>DFALPINFGADIEYTTGANSVPFEVVTNPEQSGINATDTKVGKVTNQGGQYEALT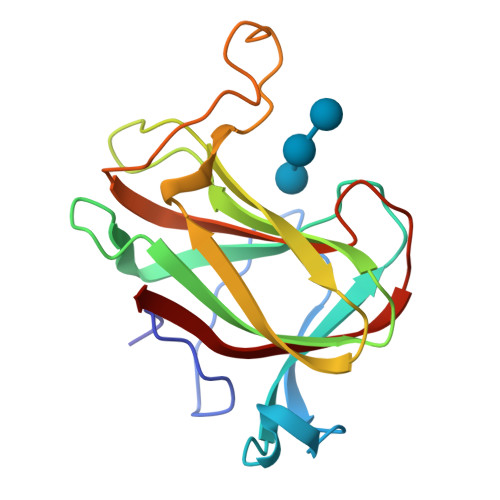FLLDEAIDFSGSNKTITMKVYSEVAYQVLFKLETGMNGERANEVEVSHSGNGWEELSFNFNNARNSFVQGDDANNGQPFVPTGQYDEISIFLDFAGFTAGDFYIDDIEQN[2x]>SNAMNVIRLKEDKFREALRLSEYAFQYKVDEDRLQQQITKMKESHEVYGIMEGENLAAKLHLIPFHIYIGKEKFKMGGVAGVATYPEYRRSGYVKELLQHSLQTMKKDGYTVSMLHPFAVSFYRKYGWELCANLLVCHMTKSDLVMKKQVNGTVKRFNKESHPEEVEKLYETFAELFSGMLVRNEKWWLQAVYDDLTLAIYYDENQTAAGYMLYKIENYKMTVEEFVPLHNEARNGLWNFICQHDSMIKDLEMTVSENEPLLYTLQEPRVKTEIKPYFMGRIV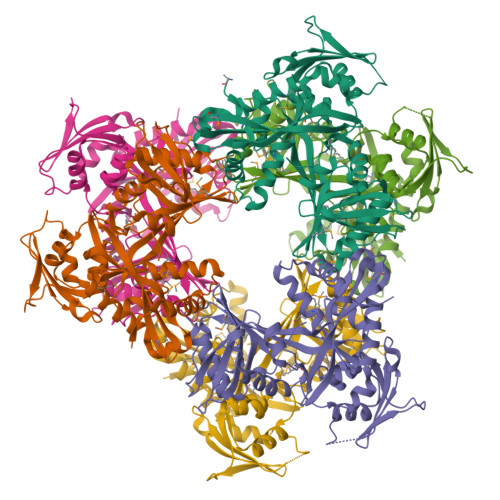DVEQFLKQYELNWNNVQQEVILHITDSFAQWNNITVRIANHEITIIEEPIDKGIKLDINALSTILFGYRRPLELNELELISGSEEEIRAFESVVPVRKPFIYDFF[6x]>MGAHSKEMAPLMGKRTTAPGGNPVVLTEKRPADLTPTKKSAHFFLEIEGFEPNPTVTKTSPPIFSKPMDSNIRQCLSGNCDDMDSPQSPQDDVTETPSNPNSPSANLAKEEQRQKKKRLKKRIFAAVSEGCVEELRELLQDLQDLCRRRRGLDVPDFLMHKLTASDTGKTCLMKALLNINPNTKEIVRILLAFAEENDILDRFINAEYTEEAYEGQTALNIAIERRQGDITAVLIAAGADVNAHAKGVFFNPKYQHEGFYFGETPLALAACTNQPEIVQLLMENEQTDITSQDSRGNNILHALVTVAEDFKTQNDFVKRMYDMILLRSGNWELETMRNNDGLTPLQLAAKMGKAEILKYILSREIKEKPLRSLSRKFTDWAYGPVSSSLYDLTNVDTTTDNSVLEIIVYNTNIDNRHEMLTLEPLHTLLHTKWKKFAKYMFFLSFCFYFFYNITLTLVSYYRPREDEDLPHPLALTHKMSWLQLLGRMFVLIWATCISVKEGIAIFLLRPSDLQSILSDAWFHFVFFVQAVLVILSVFLYLFAYKEYLACLVLAMALGWANMLYYTRGFQSMGMYSVMIQKVILHDVLKFLFVYILFLLGFGVALASLIEKCSKDKKDCSSYGSFSDAVLELFKLTIGLGDLNIQQNSTYPILFLFLLITYVILTFVLLLNMLIALMGETVENVSKESERIWRLQRARTILEFEKMLPEWLRSRFRMGELCKVADEDFRLCLRINEVKWTEWKTHVSFLNEDPGPIRRTADLNKIQDSSRSNSKTTLYAFDELDEFPETSVLVPRGSAAAWSHPQFEK[4x]

TRPV3 is a cation-permeable TRP channel predominantly expressed in skin keratinocytes, implicated in cutaneous sensation and associated with numerous skin diseases. TRPV3 dysfunction has been associated with numerous skin diseases, including atopic dermatitis, dermal fibrosis, rosacea, and itch, as well as channelopathies like Olmsted syndrome, caused by a growing list of ‘gain-of-function’ mutations. TRPV3 is inhibited by the local anesthetic dyclonine, traditionally used for topical applications to relieve pain and itch. The structure includes an ion channel, which is formed by the transmembrane domains (TMDs) of the four individual subunits, each contributing the S1–S4 and pore domains in a domain-swapped arrangement, and a large intracellular skirt that is mostly formed by the ankyrin-repeat domains (ARDs).

We used cryo-EM to solve the structure of TRPV3 in complex with dyclonine, TRPV3Dyc. Three-dimensional reconstruction with four-fold rotational symmetry (C4) resulted in a TRPV3Dyc map with overall resolution of 3.16 Å. For each subunit in the TRPV3Dyc homotetramer we built an accurate model of residues 118–756, excluding the regions of S1–S2 (residues 462–470) and S5-P (residues 611–621) loops that were not resolved clearly in the cryo-EM density. The overall architecture of TRPV3Dyc is similar to the previously solved TRPV3 structures. We found that dyclonine binds to sites inside the portals which connect the membrane environment to the central cavity of the ion channel pore. These sites are formed by the transmembrane helices S5 and S6 and have not been previously shown to bind TRPV3 inhibitors. To make room for dyclonine in the portal, the side chain of F666 flips around by about 90 degrees and its benzyl group becomes nearly parallel to the piperidine group of dyclonine. While other residues in S5 and S6 that surround dyclonine in TRPV3 maintain similar conformations as in the closed apo state, the flipped up side chain of F666 causes a shift of the P-loop away from the portal, toward the extracellular space. This conformational change does not propagate to the channel gate, which is formed by the S6 helices bundle crossing and maintains a similar conformation as in the closed state. However, we think that it is more likely that dyclonine inhibits TRPV3 by binding in the side portals and protruding into the TRPV3 pore’s central cavity, thus creating an additional barrier for ion permeation.>QTSCDQWATFTGNGYTVSNNLWGASAGSGFGCVTVVSLSGGASWHADWQWSGGQNNVKSYQNSQIAIPQKRTVNSISSMPTTASWSYSGSNIRANVAYDLFTAANPNHVTYSGDYELMIWLGKYGDIG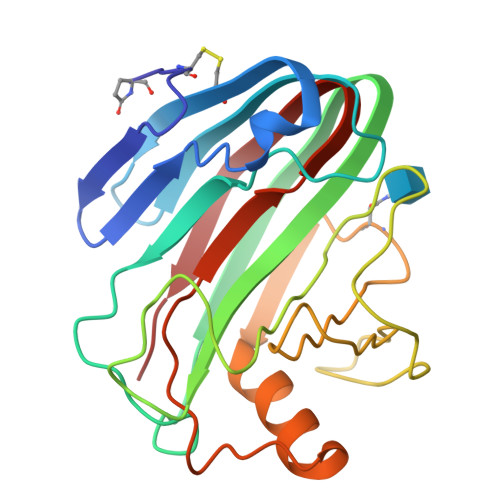PIGSSQGTVNVGGQSWTLYYGYNGAMQVYSFVAQTNTTNYSGDVKNFFNYLRDNKGYNAAGQYVLSYQFGTEPFTGSGTLNVASWTASIN[6x]RNA in all cellular organisms is synthesized by a complex molecular machine, the DNA-dependent RNA polymerase (RNAP). In bacteria, the catalytically competent core RNAP (subunit composition α2ββ'ω) has a molecular mass of ∼400 kDa. The Eco and Thermus β and β' subunits harbor large sequence insertions (>40 amino acids) that are not present in the other species and are not shared across bacterial species.

We prepared a construct comprising the Eco β2 domain including βi4 inserted within it (Eco β residues 152–443, hereafter called Eco β2-βi4). After reductive methylation, the protein formed crystals that diffracted X-rays to 1.6 Å-resolution. As expected, the Eco β2 (Eco β residues 151–224 and 344–445) and the Thermus β2 (Taq or Tth β residues 138–325) domains have similar overall structures. The βi4 domain is inserted at the surface of the β2 domain distal to the connection with the RNAP. A 3-residue segment of Taq β (Taq β 212–214) is replaced by the 119-residue Eco βi4. The Eco βi4 folds into a compact, cylinder-shaped domain about 22 Å in diameter and about 50 Å in length. The compact domain is connected to the β2 domain by two short connector loops (Eco β 225–226 and 337–345). The βi4 domain packs against β2, resulting in the burial of a modest 618 Å2 of surface area. As predicted, the Eco βi4 includes two tandem BBM2 motifs. Moreover, the solvent-exposed surface of βi4, including the entire surface facing the DNA, is highly acidic (front view), except for a “neutral patch” that arises from three conserved residues, Eco β R268, R272, and R275 (top view).

> GHPMSPGVFFDSDKGKTHSSGKVLYNARIIPYRGSWLDFEFDPKDNLFVRIDRRRKLPATIILRALNYTTEQILDLFFEKVIFEIRDNKLQMELVPERLRGETASFDIEANGKVYVEKGRRITARHIRQLEKDDVKLIEVPVEYIAGKVVAKDYIDESTGELICAANMELSLDLLAKLSQSGHKRIETLFTNDLDHGPYISETLRVDPTNDRLSALVEIYRMMRPGEPPTREAAESLFENLFFSEDRYDLSAVGRMKFNRSLLREEIEGSGILSKDDIIDVMKKLIDIRNGKGEVD>MHAALTPLTNKYRFIDVQPLTGVLGAEITGVDLREPLDDSTWNEILDAFHTYQVIYFPGQAITNEQHIAFSRRFGPVDPVPILKSIEGYPEVQMIRREANESSRFIGDDWHTDSTFLDAPPAAVVMRAIEVPEYGGDTGFLSMYSAWETLSPTMQATIEGLNVVHSATKVFGSLYQATNWRFSNTSVKVMDVDAGDRETVHPLVVTHPVTGRRALYCNQVYCQKIQGMTDAESKSLLQFLYEHATKFDFTCRVRWKKDQVLVWDNLCTM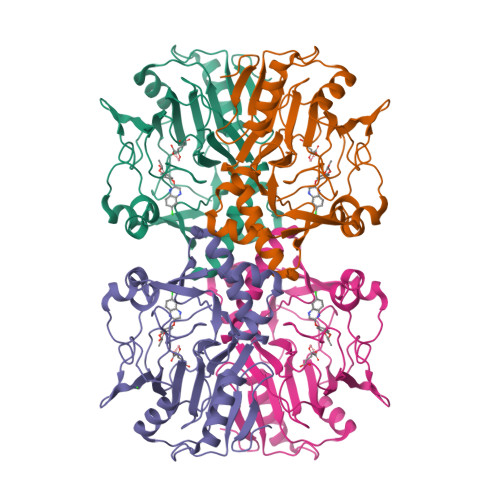HRAVPDYAGKFRYLTRTTVAGDKPSR[4x]>XMFIVNTNVPRASVPDGFLSELTQQLAQATGKPPQYIAVHVVPDQLMAFGGSSEPCALCSLHSIGKIGGAQNRSYSKLLCGLLAERLRISPDRVYINYY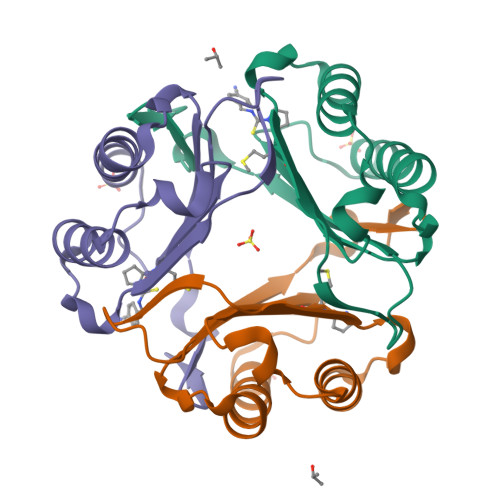DMNAANVGWNNSTFA[3x]> LEVLFQGPLGSPEFPGRLERPHMTAIAPVITVDGPSGAGKGTLCKALAESLNWRLLDSGAIYRVLALAALHHQVDISTEEALVPLAAHLDVRFVSQNGQLQVILEGEDVSNEIRTETVGNTASQAAAFPRVREALLRRQRAFREAPGLIADGRDMGTIVFPDAPVKIFLDASSQERAHRRMLQLQERGFNVNFERLLAEIQERDNRDRNRSVAPLVPAADALVLDSTSMSIEQVIEQALAYAQRILALPLKK

Cytidine monophosphate (CMP) kinase is a member of the nucleoside monophosphate (NMP) kinase family, and plays a crucial role in biosynthesis of nucleoside precursors. In bacteria, CMP kinase catalyses the transfer of a phosphoryl group from ATP to CMP or dCMP. We have elucidated the crystal structure of CMP kinase from Y. pseudotuberculosis and validated the function of the enzyme as a kinase. Yersinia CMP kinase adopts the same overall fold as related CMP kinases and is composed of nine α-helices and seven β-strands connected by loops.

There is one CMP kinase molecule in the crystallographic asymmetric unit, and the solvent content is 48 per cent. Clear density is observed from Met1 through Ala225 with the exception of a 12-residue gap from Glu180 to Ala191. The central portion of the molecule is composed of a central β-sheet, made up from β1, β2, β5, β6 and β7, and α1 and α9. The NMP-binding domain is composed of anti-parallel β-strands (β3 and β4) and helices (α2, α3, α4 and α5). Yersinia CMP kinase can be described as a member of the class of long-NMP kinases owing to the insert found in the NMP-binding domain, which is not present in short variants: in this structure, the insert comprises the anti-parallel β-strands, a loop region that connects β4 to β4, and α5. The lid domain is composed of helices α7 and α8. The ligand-binding site is formed by a pocket on the NMP-binding domain. One sulphate ion is bound at this site. The sulphate ion occupies the same position as that of previously published bacterial CMP kinase structures that have been crystallized in the absence of ATP.Growth factor receptor-bound protein 7 (Grb7) is an adaptor protein involved in cell signaling where it interacts with a number of tyrosine kinases via its src-homology2 (SH2) domain78. In this way it plays a role in integrin dependant cell migration via its interaction with focal adhesion kinase and subsequent phosphorylation in focal contacts, consistent with its homology to the C. Elegans protein Mig-10 that is involved in cellular migration. It has been shown that overexpression of Grb7 enhances cell migration, while inhibition of Grb7 lowers the migratory potential of cells and is therefore linked with metastatic spread of cancer cells. While co-overexpression of Grb7 and ErbB2 occurs due to the proximity of their two genes on the 17q12-21 amplicon, Grb7 plays a role independent of ErbB2 in cancer progression. These important roles of Grb7 in numerous cancers have established Grb7 as a therapeutic target. Following the conventional nomenclature for SH2 domains, the Grb7-SH2 domain possesses a 3 stranded anti-parallel β-sheet consisting of the βB, βC and βD strands, flanked by 2 α-helices, αA and αB.

To determine whether the fully formed staple (rather than just the O-allylserine functionalities) is required for the high affinity binding to the Grb7-SH2 domain we synthesized the G7-B4NS peptide (for G7-Bicyclic 4 No Staple) which included the thioether linkage to achieve cyclisation but was not subjected to ring-closing metathesis to form a staple via O-allyl substituted serine residues. The dissociation constant determined for G7-B4NS binding to Grb7-SH2 was KD = 4.9 μM. To investigate the observation that the ring-closed G7-B4 peptide bound with 6 fold higher affinity than the G7-B4NS peptide that had not been subjected to ring-closing metathesis, we determined the structure of the Grb7-SH2/G7-B4NS complex using X-ray crystallography, to 2.6 Å resolution. The asymmetric unit consists of four Grb7-SH2 domains (consisting of residues 429–527), two G7-B4NS peptides, 3 water molecules, and two phosphate anions. Additionally the Y5 of G7-B4NS forms analogous interactions to the Y5 of G7-B1 with the phosphate anion positioned in the pY binding pocket. Likewise, the G7-B4NS peptide residues 2–7 all form the same interactions with Grb7-SH2 as observed in the G7-B4 co-crystal structure. Electron density for the peptide, however, was not visible for the O-allylserine sidechains (and, in one molecule within the asymmetric unit, was not visible for the N-terminal two residues and, in the other molecule, not seen for the C-terminal cysteine). This absence of electron density suggests these groups are flexible and do not form an interaction with the surface of the Grb7-SH2 domain. There was also an absence of electron density for the thioether linker indicating that this linker is more flexible in this crystal form or in complex with Grb7-SH2 than the equivalent thioether linker observed in G7-B4.

>[4x]GSPASGTSLSAAIHRTQLWFHGRISREESQRLIGQQGLVDGLFLVRESQRNPQGFVLSLCHLQKVKHYLILPSEEEGRLYFSMDDGQTRFTDLLQLVEFHQLNRGILPCLLRHCCTRVAL;>SFEGYDNSC[2x]> MTKYQGYDVTDATHKTSIHNDWKVVVAKKKPARGVTLTIGIFFDGTGNNRENTASRLMKFNECSAARQGVNQKDAQSCEDFLKEINKNSISNGSYRGYYSNIHWLNILYHPDQVLKKDQTSAQIKTYISGIGTAAGEADSVIGMGLGTSILDIFEGVVTKTDEAMERITQALSEFMGFNLSPDFCIAKIQFDVFGFSRGAAAARHFANRVMEQDPAIARAIAKGLRGDFYDGKPSGEVRFLGLFDTVAAIGGISNFFDINGRSNPGVKLELRPSVAKKVFQITAMNEYRYNFSLNSIKGMWPELALPGAHSDIGGGYNPVGSPLQENESLFLSCPEFEIVSDDTREMDTRVYRKAEQVRKMLMTLPALKHILPHGKLTTKIRSIGVNNSNQRRAGVIQKQVGAAVFFERMAVPNDWANVCLRVMLDAAQEAGVLFEPIRQTNTELQLPSELIF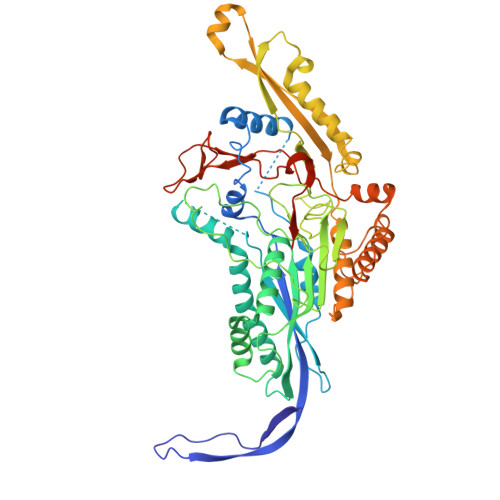LADKAIAQGKAVRLGQEPQAFTEEELYIIGKYTHCSANWNIESDGNLWVDPTTGEIFIHRFGPKGNKAFVFPNKPNDRWIRSVWYMDDQQRLNDNAVKNTKVMMSGV(2R)-2-[(1R)-1-{[(2R)-2-carboxy-2-(4-hydroxyphenyl)acetyl]amino}-1-methoxy-2-oxoethyl]-5-methylidene-5,6-dihydro-2H-1,3-oxazine-4-carboxylic acid | C18 H18 N2 O9 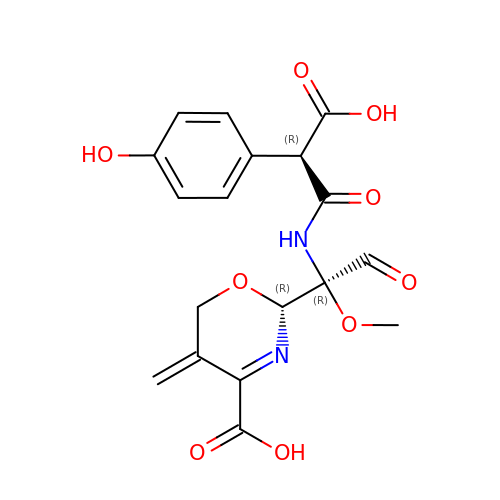| GOYCBKVVHGALFQ-PJSAGSTRSA-N> EQGGFSGPSA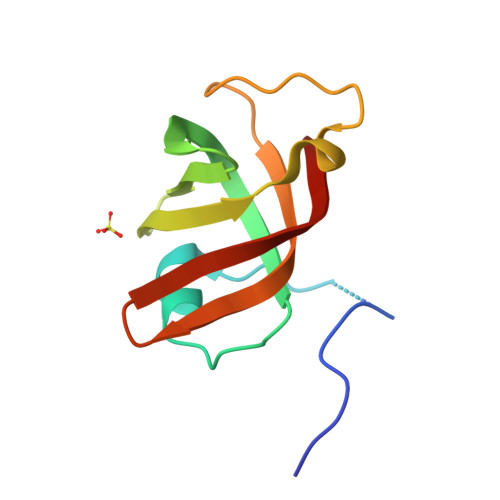TQSQAGGFQGPNGSVTTVESAKSLRDDTWVTLRGNIVERISDDLYVFKDASGTINVDIDHKRWNGVTVTPKDTVEIQGEVDKDWNSVEIDVKQIRKVNP> GDEESGKADRAYKPIEIYGNINEVVNNVQETRAVGAAWGSDDRIGVTVEADEDNATANAVDTYINIQYRNETGGSFRVVNEGSTDNNIRLKGEGEFTLNAYYPYQGANGTLPGTEGVIAKTISGADQTTDKQPQIDFLFAQATGVRAESPVTFDFSHKMTKIILKFKATNGATLNNMKVYLKSLQLEGSFNVTTGEAVAKSGATPNSELSMDIAKPAEGEMTASIILFPQDMPEKVLLEVRMNDETYTQYMPVQN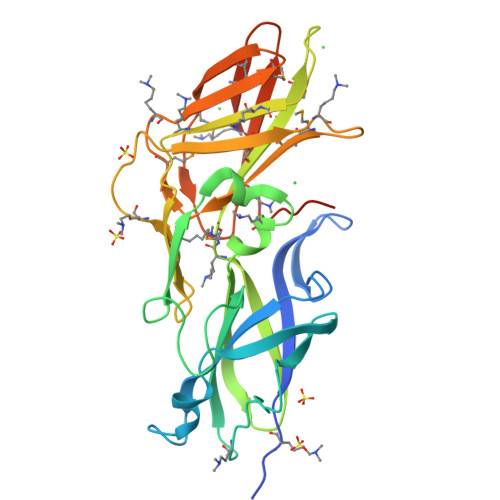LESGHAYPYNVTFENPAMTITKAEIEDWIVEDDKDVTASVTE> MHHHHHHMPLEPHFMPDFLGH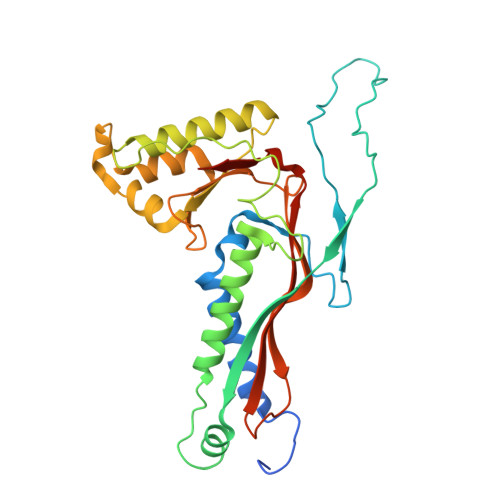AENPLREEEWARLNETVIQVARRSLVGRRILDIYGPLGAGVQTVPYDEFQGVSPGAVDIVGEQETAMVFTDARKFKTIPIIYKDFLLHWRDIEAARTHNMPLDVSAAAGAAALCAQQEDELIFYGDARLGYEGLMTANGRLTVPLGDWTSPGGGFQAIVEATRKLNEQGHFGPYAVVLSPRLYSQLHRIYEKTGVLEIETIRQLASDGVYQSNRLRGESGVVVSTGRENMDLAVSMDMVAAYLGASRMNHPFRVLEALLLRIKHPDAICTLEGAGATERR>[4x]MASWSHPQFEKGAETAVPNSSSVPGDPSSMTRKNVLLIVVDQWRADFIPHLMRAEGREPFLKTPNLDRLCREGLTFRNHVTTCVPGGPARASLLTGLYLMNHRAVQNTVPLDQRHLNLGKALRAIGYDPALIGYTTTTPDPRTTSARDPRFTVLGDIMDGFRSVGAFEPNMEGYFGWVAQNGFELPENREDIWLPEGEHSVPGATDKPSRIPKEFSDSTFFTERALTYLKGRDGKPFFLHLGYYRPHPPFVASAPYHAMYKAEDMPAPIRAENPDAEAAQHPLMKHYIDHIRRGSFFHGAEGSGATLDEGEIRQMRATYCGLITEIDDCLGRVFAYLDETGQWDDTLIIF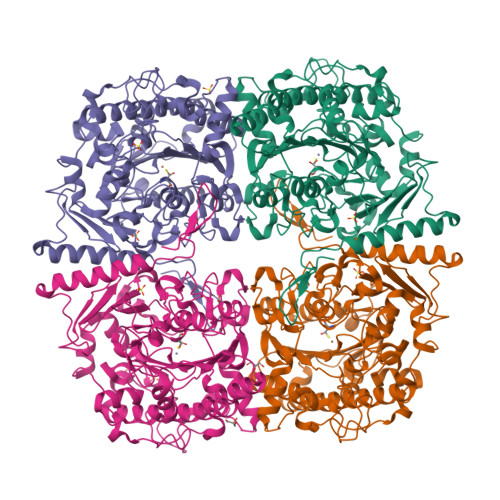TSDHGEQLGDHHLLGKIGYNAESFRIPLVIKDAGQNRHAGQIEEGFSESIDVMPTILEWLGGETPRACDGRSLLPFLAEGKPSDWRTELHYEFDFRDVFYDQPQNSVQLSQDDCSLCVIEDENYKYVHFAALPPLFFDLKADPHEFSNLAGDPAYAALVRDYAQKALSWRLSHADRTLTHYRSSPQGLTTRNH> MKNTPQHKLFFVVALLLVVQILAGCKSSSSTTAGSTENSSSSTPDPDTGTTTPDPIEPEVVPPVTPPSVDSNSREVIPLWEDKVADGKAWSTHVYSALDKLGPNLLDVIPADRSLFCPKYSSLSYAQRKQYWAFVLSSMVRFQSNFKTAMSYTEDFNDSNGNRVISRGLLQISIESGNAYGCGFKSTKDLHDPLQNLSCGIRILDRWVSRDGRIAGKVDGAWKGGARYWSVLRAGDKTSYKSIVSWSQNLSICK

Here, we discover a family of Bdellovibrio proteins that define a new subgrouping of the lysozyme superfamily and demonstrate that they possess outright specificity for deacetylated peptidoglycan. We solve the structure of family member Bd0314 (that we named DslA), revealing adaptations to the lysozyme fold that sterically restrict the active-site cleft into only accepting polymers deacetylated at the GlcNAc positions. We determine a role for DslA in B. bacteriovorus exit from the prey cell and demonstrate that exogenously added enzyme is able to prematurely liberate predators from prey bdelloplasts before completion of the predatory lifecycle. The architecture of DslA is related to, but significantly different from, other members of the lysozyme superfamily but still fulfil the inclusion criteria for the lysozyme superfamily noted by Monzingo et al. — conservation of the β-sheet floor and helices D and F, with appropriate placement of acidic catalytic residues.

Using the DslA structure as a guide, we next monitored the activity of DslA mutants for the putative active-site residues. Variants E143Q and E154Q clearly fold and retain a similar active-site architecture (as judged by our high-resolution structures herein), but display no notable activity (middle), confirming their participation in catalysis. The lysozyme superfamily has a conserved ES motif at the C terminus of a central α-helix, which is readily identifiable as E143/S144 on DslA helix D. Residue E143 of the conserved ES motif would act as a general acid, protonating the equatorial linkage between MurNAc and GlcN, with E154 acting as a general base to activate water to attack the MurNAc C1 in an axial orientation. The structural equivalence of DslA E154 to the β1 secondary catalytic acid residues of goose-type lysozymes (also GH23, but with a second catalytic residue lacking in the lytic transglycosylases), v-type lysozymes and chitosanases, and our assay on the E143Q and E154Q mutants argues for an inverting hydrolytic mechanism for DslA. All four of our DslA structures (two wild-type, E143Q, E154Q) are highly similar, other than a relatively small flexation of the β1–2 hairpin in the E154Q variant. Additional controls were performed using EDTA plus DslA with one of the catalytic site residues inactivated (E143Q), or using conventional hen egg-white lysozyme (HEWL) or buffer only. The percentage of prematurely released, external predator cells increased significantly when early bdelloplasts were treated by exogenous addition of DslA, whereas no significant change was detected for the treatment controls DslA E143Q, HEWL or buffer only.>[2x]MVMLHSKNVKGFLENTLKPYGSLQSSMIITATNGGILSYATSNNDVPKNSINEINSVNNLKMMSLLIKDKWSEDENDTEEQH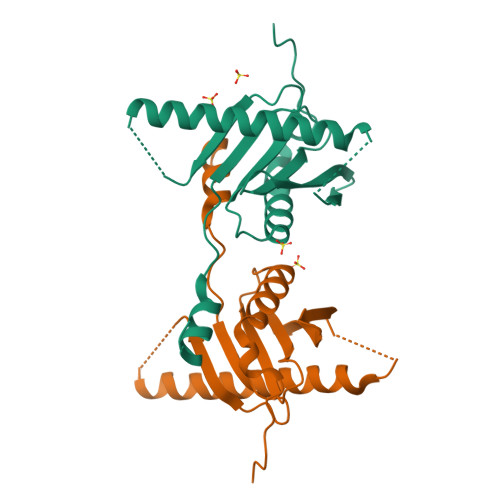SNSCYPVEIDSFKTKIYTYEMEDLHTCVAQIPNSDLLLLFIAEGSFPYGLLVIKIERAMRELTDLFGYKLGLEHHHHHH8-HYDROXYCOUMARIN 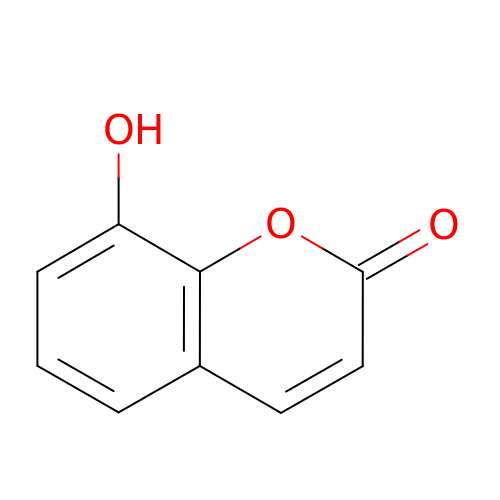| C9 H6 O3 | DPTUTXWBBUARQB-UHFFFAOYSA-N> GGSMEFSGRKWRKLRLAGDQRNASY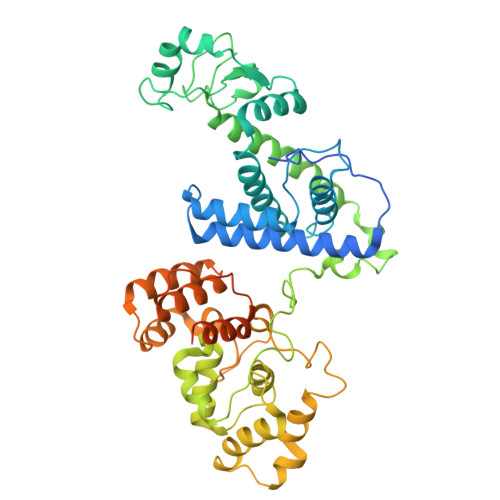PHCLQFYLQPPSENISLIEFENLAIDRVKLLKSVENLGVSYVKGTEQYQSKLESELRKLKFSYRENLEDEYEPRRRDHISHFILRLAYCQSEELRRWFIQQEMDLLRFRFSILPKDKIQDFLKDSQLQFEAISDEEKTLREQEIVASSPSLSGLKLGFESIYKIPFADALDLFRGRKVYLEDGFAYVPLKDIVAIILNEFRAKLSKALALTARSLPAVQSDERLQPLLNHLSHSYTGQDYSTQGNVGKISLDQIDLLSTKSFPPCMRQLHKALRENHHLRHGGRMQYGLFLKGIGLTLEQALQFWKQEFIKGKMDPDKFDKGYSYNIRHSFGKEGKRTDYTPFSCLKIILSNPPSQGDYHGCPFRHSDPELLKQKLQSYKISPGGISQILDLVKGTHYQVACQKYFEMIHNVDDCGFSLNHPNQFFCESQRILNGGKDIKKEPIQPETPQPKPSVQKTKDASSALASLNSSLEMDMEGLEDYFSEDS>[4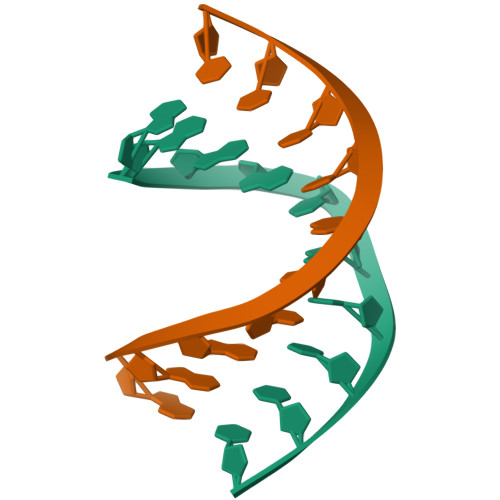x]GGGGCGCCCC>[2x]VTYPGAIPLSLTSNYETPSPTAIPLEPTPTATGTAELDALWNLVEAQYPVQTAAVTTLVTVPDDYKFE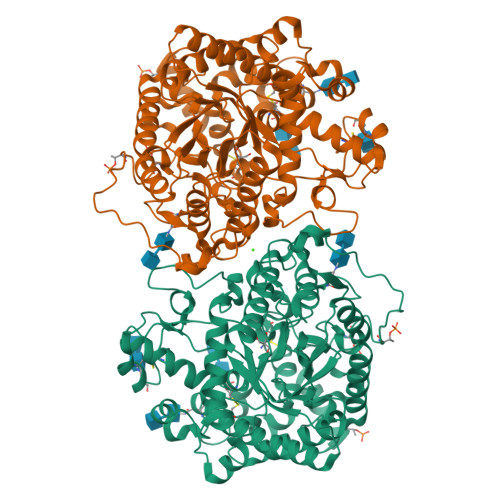ADPPSYALAGYETSEIAGLKFPKGFKFGVAGAAIQVEGAAKAEGRGPSTWDYLCHHYASTQCNNYDPDITTNHYYLYPLDFARLQHLGINTYSFSISWTRIYPLGAGYVNEAGLAHYDAVIHSAKKYGLEPVGTVFHWDTPLSLMLKYGAWQDTGDQIVKDFVTYATTVFKRYGNEVKTWFTFNEPRVFCSQNSGLPYNLTYPEGINSTSAVFRCTYNVLKAHGHAVKVYRDLVASGTIAAGEIGFKSDDNYPIPARPGNADDEESAKRHEAFRIGIFAQPVYGNGDYPDVVKETVGDMLPALTDEDKGYIKGSGDIFAIDGYRTDISHAALNGIANCIRNQSDPNWPVCEEGSDPFAHVYPSGFAIGQSADPLSSWLVNSAPFIRDQLKFLTQTYPAKGGIYFSEFGWAEDAEYDRQLLYQITWDGLRTQYLTDYLSQLLLAVHKDGINLRGALTWSFVDNWEWGLGMQQKFGFQFVNQSDPDLTRTFKLSAHAYAQFGRNHLHHHHHH> GHACPSQCSCDQTTVKCHSRRLTSVPAGIPTTTKILRLYSNQITKLEPGVFDHLVNLEKLYISWNQLSALPVGVFDKLTKLTHLSLGYNQLKSVPRGAFDNLKSLTHIWLLNNPWDCECSDILYLKN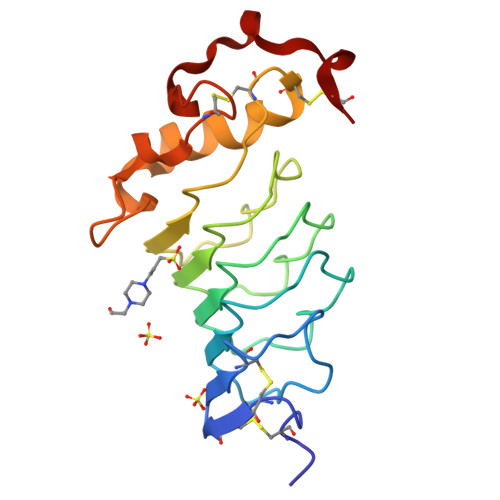WIVQHASIVNLQGHGGVDNVKCSGTNTPVRAVTEASTSPSKCP>[2x]EQTYYDLVKAFMAEIRQYIRELNLIIKVFREPFVSNSKLFSANDVENIFSRIVDIHELSVKLLGHIEDTVEMTDEGSPHPLVGSCFEDLAEELAFDPYESYARDILRPGFHDRFLSQLSKPGAALYLQSIGEGFKEAVQYVLPRLLLAPVYHCLHYFELLKQLEEKSEDQEDKECLKQAITALLNVQSGMEKICSKSLAKRRLSESACRFYSQQMKGKQLAIKKMNEIQKNIDGWEGKDIGQCCNEFIMEGTLTRVGAKHERHIFLFDGLMICCKSNHGQPRLPGASNAEYRLKEKFFMRKVQINDKDDTNEYKHAFEIILKDENSVIFSAKSAEEKNNWMAALISLQYRSTLERMLDVTMLQEEKEEQMRLPSADVYRFAEPDSEENIIFEENMQPKAGIPIIKAGTVIK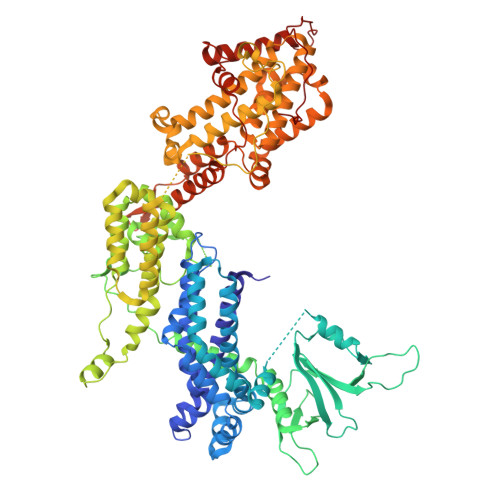LIERLTYHMYADPNFVRTFLTTYRSFCKPQELLSLIIERFEIPEPEPTEADRIAIENGDQPLSAELKRFRKEYIQPVQLRVLNVCRHWVEHHFYDFERDAYLLQRMEEFIGTVRGKAMKKWVESITKIIQRKKIARDNGPGHNITFQSSPPTVEWHISRPGHIETFDLLTLHPIEIARQLTLLESDLYRAVQPSELVGSVWTKEDKEINSPNLLKMIRHTTNLTLWFEKCIVETENLEERVAVVSRIIEILQVFQELNNFNGVLEVVSAMNSSPVYRLDHTFEQIPSRQKKILEEAHELSEDHYKKYLAKLRSINPPCVPFFGIYLTNILKTEEGNPEVLKRHGKELINFSKRRKVAEITGEIQQYQNQPYCLRVESDIKRFFENLNPMGNSMEKEFTDYLFNKSLEIEPRNPKPLPRFPKKYSYPLKSPGVRPSNPRPGT> ASLTEIEHLVQSVCKSYRETCQLRLEDLLRQRSNIFSREEVTGYQRKSMWEMWERCAHHLTEAIQYVVEFAKRLSGFMELCQNDQIVLLKAGAMEVVLVRMCRAYNADNRTVFFEGKYGGMELFRALGCSELISSIFDFSHSLSALHFSEDEIAL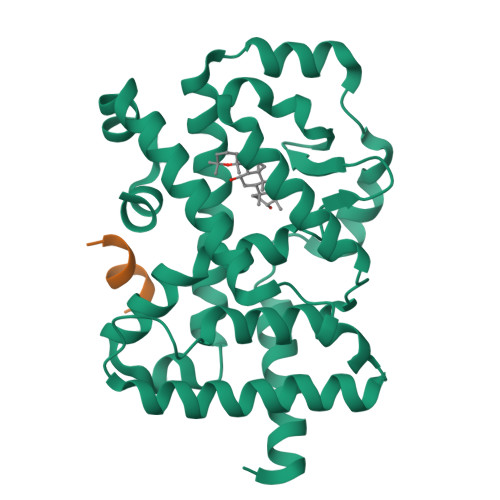YTALVLINAHRPGLQEKRKVEQLQYNLELAFHHHLCKTHRQSILAKLPPKGKLRSLCSQHVERLQIFQHLHPIVVQAAFPPLYKELFS;> KILHRLLQ The structure-specific nuclease, flap endonuclease-1 (FEN1) plays a vital role in maintaining genome integrity by precisely processing intermediates of Okazaki fragment maturation, long-patch excision repair, telomere maintenance, and stalled replication forks. FEN1 preferentially binds to double flap substrates with a one nt 3′-flap and any length of 5′-flap, including zero. It catalyses a single hydrolytic incision one nucleotide (nt) into dsDNA to yield nicked DNA ready for direct ligation. Here crystallographic analyses uncover an unprecedented electrostatic steering of an inverted 5′-flap through the human FEN1 (hFEN1) helical gateway.

To obtain structures of hFEN1 with a ss 5′-flap substrate for insight into ss 5′-flap selection, we crystallized three hFEN1 active site mutants D86N, R100A and D233N with a double-flap (DF) substrate and with Sm3+. The third independent hFEN1-D233N crystal structure captures two cleaved nts from the 5′-flap bound on the other side of the tunnel from the dsDNA, consistent with threading. Asp233 is 3 Å from the attacking water and contributes modestly to catalysis; the D233N mutant has 16-fold reduced but still substantial catalytic activity compared to mutants of other invariant carboxylates, such as D181A21 and D86N. D86N, R100A and D233N mutations slow the hFEN1 catalysed reaction rate by factors of 530, 7,900 and 16 respectively. An ordered gateway and cap formed by helices 2, 4 and 5 are observed above the active site in these three structures. In all three substrate structures, the dsDNA major groove is widened as it approaches the active site, and DNA bases flanking the scissile phosphate are stacked with one another, with the +1 base packed against Tyr40.

> GIQGLAKLIADVAPSAIRENDIKSYFGRKVAIDASMSIYQFLIAVRQGGDVLQNEEGETTSHLMGMFYRTIRMMENGIKPVYVFDGKPPQLKSGELAKRSERRAEAEKQLQQAQAAGAEQEVEKFTKRLVKVTKQHNDECKHLLSLMGIPYLDAPSEAEASCAALVKAGKVYAAATEDMDCLTFGSPVLMRHLTASEAKKLPIQEFHLSRILQELGLNQEQFVDLCILLGSNYCESIRGIGPKRAVDLIQKHKSIEEIVRRLDPNKYPVPENWLHKEAHQLFLEPEVLDPESVELKWSEPNEEELIKFMCGEKQFSEERIRSGVKRLSKSRQGSTLEVLFQ Membrane-bound pyrophosphatases are homodimeric integral membrane proteins that hydrolyze pyrophosphate into orthophosphates, coupled to the active transport of protons or sodium ions across membranes. They are important in the life cycle of bacteria, archaea, plants, and parasitic protists, but no homologous proteins exist in vertebrates, making them a promising drug target. In all these structures, mPPase is a symmetric homodimer, with each monomer consisting of 16 TMHs. Each monomer consists of four regions: a hydrolytic center, a coupling funnel, an ion gate, and an exit channel.

Here, we report the discovery and synthesis of the first nonphosphorus, non–substrate-analog inhibitor of TmPPase, N-[(2-amino-6-benzothiazolyl)methyl]-1H-indole-2-carboxamide (ATC), its preliminary structure-activity relationships (SARs), and a 3.4 to 4.0 Å resolution structure of ATC bound to TmPPase. Molecular replacement identified four TmPPase molecules (two dimers) in the asymmetric unit. However, only one ATC (ATC-3) could be located at the interface between chains B and C as the density in these chains was weaker. The overall structure of the TmPPase:IDP:ATC complex is very similar to that of the TmPPase:IDP complex, with an RMSD/Cα of 0.50 and 0.43 Å to dimers AB and CD, respectively. In addition, at the gate of the TmPPase:IDP:ATC structure, Na+ is pentacoordinated by D2436.50, E2466.53, S2476.54, and D70316.46 (bidentate to both carboxylate oxygens). In TmPPase:IDP, the coordinating residues are D2436.50 (side chain and main chain), E2466.53, S2476.54, and D70316.46, and the D2436.50 C═O─Na+ distance is 2.8 Å versus the considerably longer 4.0 Å in TmPPase:IDP:ATC. This is mostly because the sodium ion appears to be translated by about ~1.7 Å. In contrast, the RMSDs/Cα for the other loops that interact with ATC is smaller. Comparing all the TmPPase states shows that the binding of ATC causes the β1–2 strand of chain A to move away from the dimer interface relative to its position in TmPPase:IDP and TmPPase:2Pi to roughly the same angle as in the resting and Pi structures (Fig. 3C, inset bottom view; periplasmic side)—when the exit channel must remain closed at all times. The movement of chain A β1–2 due to the binding of the ATC dimer thus creates a hydrophobic clamp that locks the TmPPase exit channel in a closed state after substrate binding. ATC is thus an uncompetitive dimeric inhibitor with a clear preference for binding to the single-substrate bound form.

>[4x]MRGSHHHHHHYVAALFFLIPLVALGFAAANFAAVVRKPEGTERMKEISSYIRSGADSFLAHETKAIFKVAIVIAILLMIFTTWQTGVAFLLGAVMSASAGIVGMKMATRANVRVAEAARTTKKIGPALKVAYQGGSVMGLSVGGFALLGLVLVYLIFGKWMGQVDNLNIYTNWLGINFVPFAMTVSGYALGCSIIAMFDRVGGGVYTKAADMAADLVGKTELNLPEDDPRNPATIADNVGDNVGDVAGLGADLLESFVGAIVSSIILASYMFPIYVQKIGENLVHQVPKETIQALISYPIFFALVGLGCSMLGILYVIVKKPSDNPQRELNISLWTSALLTVVLTAFLTYFYLKDLQGLDVLGFRFGAISPWFSAIIGIFSGILIGFWAEYYTSYRYKPTQFLGKSSIEGTGMVISNGLSLGMKSVFPPTLTLVLGILFADYFAGLYGVAIAALGMLSFVATSVSVDSYGPIADNAGGISEMCELDPEVRKITDHLDAVGNTTAAIGKGFAIGSAIFAALSLFASYMFSQISPSDIGKPPSLVLLLNMLDARVIAGALLGAAITYYFSGYLISAVTKAAMKMVDEIRRQAREIPGLLEGKAKPDYNRCIEITSDNALKQMGYPAFIAILTPLVTGFLLGAEFVGGVLIGTVLSGAMLAILTANSGGAWDNAKKYLEAGNLEGYGKGSEPHKALVIGDTVGDPLKDTVGPSLDILIKIMSVVSVIAVSIFKHVHLF>MAVLAESELGSEAQRERRKRILDATMAIASKGGYEAVQMRAVADRADVAVGTLYRYFPSKVHLLVSALGREFSRIDAKTDRSAVAGATPFQRLNFMVGKLNRAMQRNPLLTEAMTRAYVFADASAASEVDQVEK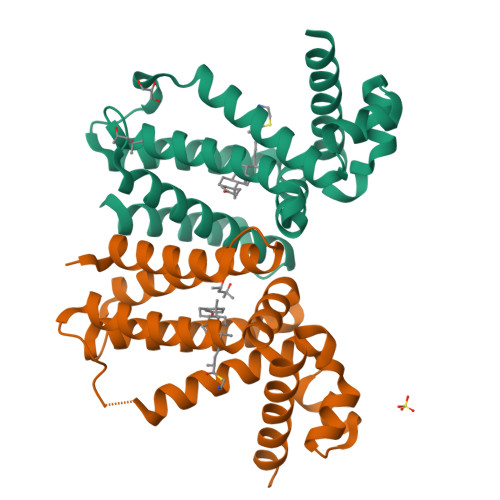LIDSMFARAMANGEPTEDQYHIARVISDVWLSNLLAWLTRRASATDVSKRLDLAVRLLIGDQDSAHHHHHH[2x]> NKSLVDQMLVELDKKISAQMDEILHNSQFQAMESAWRGLKLFVDRTDFRENNKVEILHVTKDELLEDFEFAPETAQSGLYKHVYSAGYGQFGGEPVGAIIGNYAFTPSTPDMKLLQYMGALGAMAHAPFISSVGPEFFGIDSFEELPNIKDLKSTFESPKYTKWRSLRESEDARYLGLTAPRFLLRVPYDPIENPVKSFNYAENVSASHEHYLWGNTAFAFATRLTDSFAKYRWCPNIIGPQSGGAVEDLPVHVFESMGALQSKIPTEVLITDRKEFELAEEGFIALTMRKGSDNAAFFSANSIQKPKVFPNTKEGKEAETNYKLGTQLPYMMIINRLAHYVKVLQREQIGAWKERQDLERELNSWIKQYVADQENPPADVRSRRPLRAARIEVMDVEGN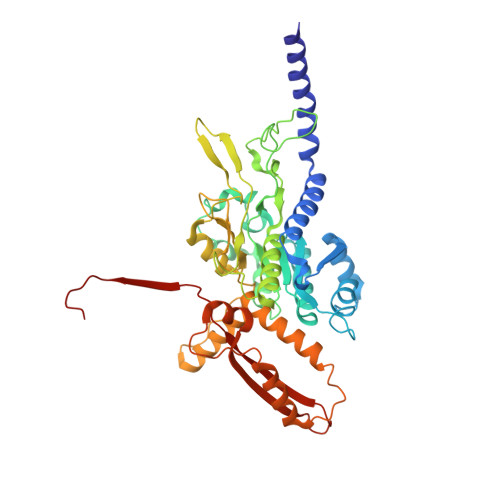PGWYQVSLSVRPHFKYMGANFELSLVGRLD2-hydroxy-3-(4-methoxybenzyl)naphthalene-1,4-dione | C18 H14 O4 | 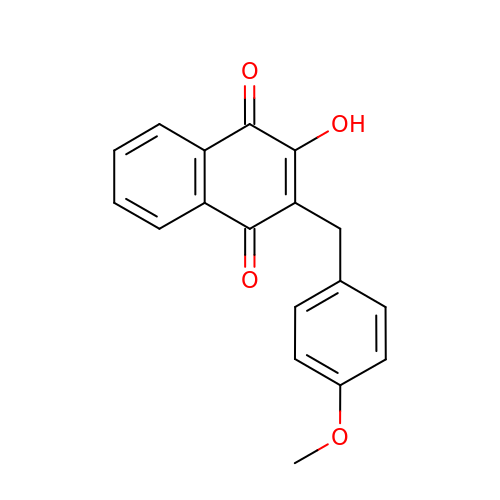DKOJAMITDVVFPR-UHFFFAOYSA-N>GPGTNRSLIVTTLLEEPFVMFRKSDRTLYGNDRFEGYCIDLLKELAHILGFSYEIRLVEDGKYGAQDDKGQWNGMVKELIDHKADLAVAPLTITHVREKAIDFSKPFMTLGVSILYRKGTPIDSADDLAKQTKIEYGAVKDGATMTFFKKSKISTFEKMWAFMSSKPSALVKNNEEGIQRT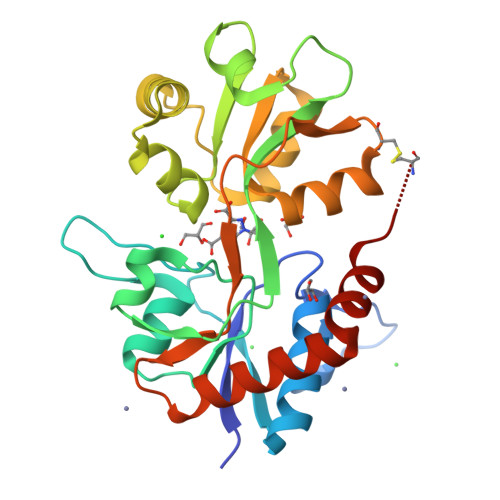LTADYALLMESTTIEYITQRNCNLTQIGGLIDSKGYGIGTPMGSPYRDKITIAILQLQEEDKLHIMKEKWWRGSGCP[2x]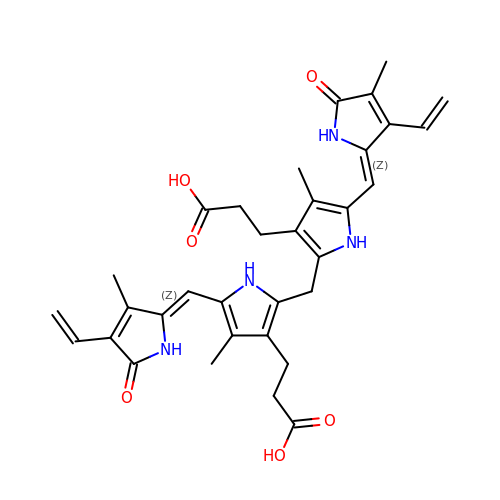3-[5-[(Z)-(4-ethenyl-3-methyl-5-oxidanylidene-pyrrol-2-ylidene)methyl]-2-[[5-[(Z)-(3-ethenyl-4-methyl-5-oxidanylidene-pyrrol-2-ylidene)methyl]-3-(3-hydroxy-3-oxopropyl)-4-methyl-1H-pyrrol-2-yl]methyl]-4-methyl-1H-pyrrol-3-yl]propanoic acid | C33 H36 N4 O6 | BPYKTIZUTYGOLE-IFADSCNNSA-N> GSSYMDVRIFEDERVDICQDLTATFISYREGPEMFRHSINLEQSSDIFRIEASGEVKHFPWMNVSELAQESAFFVEQERFVYEYIMNVFKAGRPVVFEYRCKFVPFECTVLQMMDGNTLTRYTVDKGVETLGSPPYSPDVSEDDIARYGQGSGISILRDNAALLQKRWTSFCRKIVAMDNPRHNEYSLYSNRGNGYVSCTMRTQVPLAYNISLANGVDIYKYMRMYSGGRLKVEAWLDLRDLNGSTDFAFVISSPTGWYATVKYSEYPQQSPGMLLSSIDGQFESSAVVSWHRGHGLKHAPPVSAEYSILVPRG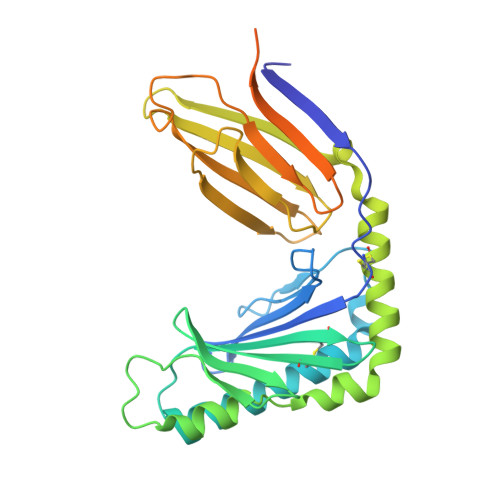SHHHHHH Jasmonates are phytohormones that are pivotal in mediating plant responses to various biotic and abiotic stresses and regulating plant growth. The first crystal structure of OPR3 from tomato (SlOPR3) showed that the enzyme crystallized as a self-inhibitory dimer in which the L6 loop, a critical loop involved in substrate recognition and coenzyme binding, from each protomer intrudes into the active site cavity of the other protomer. Based on these observations, it was postulated that the formation of the self-inhibitory homodimer represents a mechanism for regulating OPR3 activity and, thereby, jasmonic acid biosynthesis.

The wild-type self-inhibitory and R283E homodimer differ mainly in their L6 conformations. The sulfate binding site of both homodimers superimposes well, but no sulfate ion is bound in the R283E-dimer structure, corroborating that the sulfate-mediated interactions are not required for dimer formation. The dimer interface in R283E seems less stable than that in the wild type because loop L6 of one protomer in R283E is highly flexible, as evidenced by the quality of the electron density map. So, substituting R283 for glutamic acid seems to destabilize loop L6 and thus the dimer. A precise comparison of the dimers suggests that the amino acid substitution disrupts interactions that stabilize the stretched conformation of L6. In the wild-type homodimer, R283 is involved in intramolecular salt bridges that—together with other salt bridges—seem to maintain the stretched conformation of both loops in the dimer (top). These R283-mediated salt bridges are missing in R283E. Instead, E283 forms a salt bridge with R343 in one protomer, which is located at the enzyme's active site entrance, thereby destabilizing the whole loop L6, as evidenced by missing electron density for large parts of the loop (bottom). However, in the second protomer, the stretched conformation of L6 is maintained, as a salt bridge between R294 and E301 and a strong H-bond between Y284 and E300 compensate for the missing R283-mediated salt bridge; E283 is not resolved in this protomer due to disorder. Considering both the DLS and crystallographic data, it seems that the amino acid substitution R283E increases the flexibility of loop L6 in the corresponding variant, impeding proper dimer formation.

>[2x]HHHHHHMASSAQDGNNPLFSPYKMGKFNLSHRVVLAPMTRCRALNNIPQAALGEYYEQRATAGGFLITEGTMISPTSAGFPHVPGIFTKEQVREWKKIVDVVHAKGAVIFCQLWHVGRASHEVYQPAGAAPISSTEKPISNRWRILMPDGTHGIYPKPRAIGTYEISQVVEDYRRSALNAIEAGFDGIEIHGAHGYLIDQFLKDGINDRTDEYGGSLANRCKFITQVVQAVVSAIGADRVGVRVSPAIDHLDAMDSNPLSLGLAVVERLNKIQLHSGSKLAYLHVTQPEYVAYGQTEAGRLGSEEEEARLMRTLRNAYQGTFICSGGYTRELGIEAVAQGDADLVSYGRLFISNPDLVMRIKLNAPLNKYNRKTFYTQDPVVGYTDYPFLQGNGSNGPLSRL>GMDVLQKEIDEVYATHPTAHEALDNGIVEQHQQFVRSLTEVNGGCAVISDLSNRKSYVTVHPWANFLG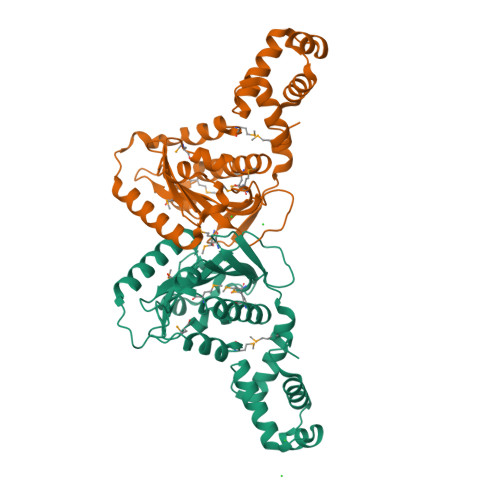LTPEEAALSVIDSMDEDCIYRRIHPEDLVEKRLMEYKFFQKTFSMSPGERLKYRGRCRLRMMNEKGVYQYIDNLVQIMQNTPAGNVWLIFCLYSLSADQRPEQGIYATITQMERGEVETLSLSEEHRNILSEREKEILRCIRKGLSSKEIAATLYISVNTVNRHRQNILEKLSVGNSIEACRAAELMKLL[3x]>[2x]MKILKDDAPELHAIAAEVPHGEDVKDLVLDMTAAMTAAGGIGLAGNQVGVLKRIIVLRCPTFKGCVINPIITRHTDGHVYSPEGCLSYPGKTVAKKRRNKVVVEGYDMDWQPITIAAKGLTAFCLQHEIDHLNGVTI

Peptide deformylases (PDFs) are enzymes involved in a pervasive and essential process called N-terminal methionine excision (NME). During NME, PDFs catalyze the removal of the formyl moiety from initiator methionine, found at the beginning of all prokaryotic translation products. We provide the first evidence that some viral PDFs, including the shortest PDF identified to date, Vp16 PDF, display deformylase activity in vivo. To conclude, characterization of the phage Vp16 PDF allows us to unexpectedly uncover the crucial role of the most unusual final amino acid in fully compensating for the 30 amino acid longer C-domain to ensure full deformylase activity.

To gain insight into the properties of these novel viral PDFs, we determined the X-ray crystal structure of Vp16 PDF. The crystal structure of the protein could be solved by molecular replacement using the structure of Pseudomonas aeruginosa PDF without its C-terminal extremity as a search model. Two crystal forms of Vp16 PDF grown under different crystallization conditions were used. Superimposition of all chains showed very similar structures (r.m.s.d. of all of Cα < 0.5 Å). The Vp16 PDF structure is composed of two α-helices (α1 and α2), two 310-helices (η1 and η2) and seven β-strands (β1 to β7) organized into two sub-domains between which lies the active site. Moreover, Vp16 PDF lacks the α3 helix usually found in Type 1B PDFs, as expected from sequence alignments. Unforeseen, Vp16 PDF is also devoid of the conserved η3 helix. Several metal cations could be identified in the structure. Particularly, a zinc cation was identified within the active site, which was coordinated similarly to other PDF structures, i.e., by Cys of motif II, the two His of motif III and one water molecule. Interestingly, the two final residues of Vp16 PDF, Thr136 and Ile137, lying very close to the active site, are involved in a network of interactions unseen in any PDF thus far.> MMKPEDVIKEQCARAKVVAELWHGFTGGAPKAALENLVVEFNKAQQGRCVRAQAAENNIALYLEAKALLPIESLGVKLQGVNLTFLNAVRFGGVVYGVPFNKSIQVLYYNKDLLKKHGVPVPATLEEFVAAAKKLSRAEGGPVYWFQPDASTFAYFFFNLGGSYLKDGKLVLNSKEAVEALTLLQNGVKEGWAKPITSGAINQNLGSGPYAFSVDTSAGYTAYLRAAKFDLGVATLPGRTKGQPGYGLVQGTNLVVFRQAS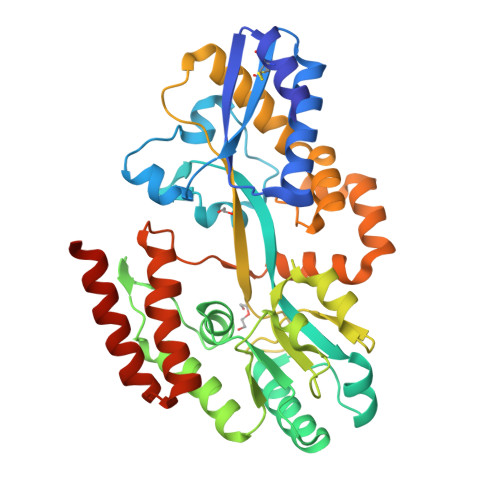KEEQAVAKDFLEFVLSPRAQAVFATATGYVPVTEGALKDPVYQAYAAENPDYATIVRQSRYAKFEPALAEWEQIRFDILGQAIKEAILNKADPKAALDRAQKLAEDLLSSRTRHHHHHH>MKPISIIGVPMDLGQTRRGVDMGPSAMRYAGVIERLERLHYDIEDLGDIPIGKAERLHEQGDSRLRNLKAVAEANEKLAAAVDQVVQRGRFPLVLGGDHSIAIGTLAGVAKHYERLGVIWYDAHGDVNTAETSPSGNIHGMPLAASLGFGHPALTQIGGYSPKIKPEHVVLIGVRSLDEGEKKFIREKGIKIYTMHEVDRLGMTRVMEETIAYLKERTDGVHLSLDLDGLDPSDAPGVGTPVIGGLTYRESHLAMEMLAEAQIITSAEFVEVNPILDERNKTASVAVALM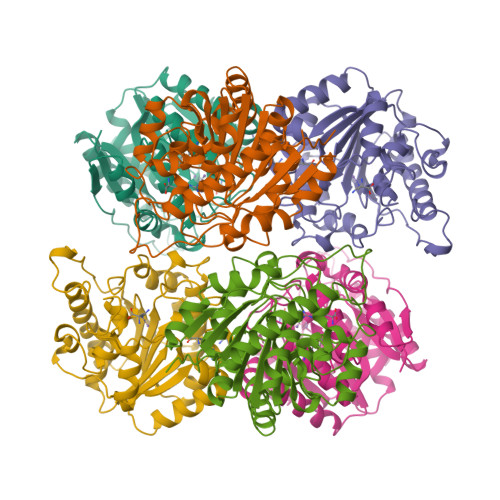GSLFGEKLM[6x]9-{5-O-[(R)-hydroxy{[(R)-hydroxy(phosphonoamino)phosphoryl]oxy}phosphoryl]-alpha-L-arabinofuranosyl}-9H-purin-6-amine 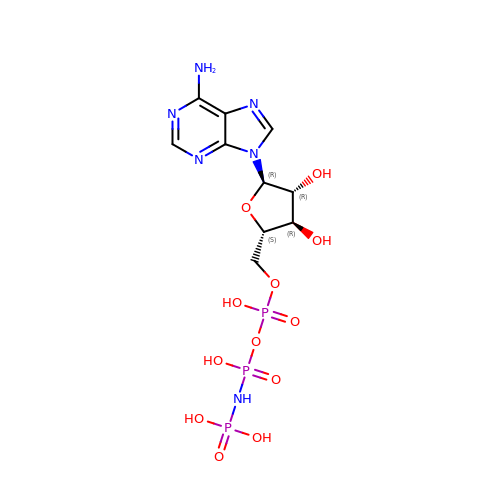| C10 H17 N6 O12 P3 | PVKSNHVPLWYQGJ-FCIPNVEPSA-N P. gingivalis displays two forms of fimbriae on its surface, FimA and Mfa1, both of which are crucial for attachment to other bacteria in the oral biofilm and to the host cells. In the work presented herein we have determined the crystal structures of the shaft protein Mfa1, in both mature and precursor forms, the anchor protein Mfa2 and a truncated precursor form of the tip protein, Mfa3. The resulting mature protein thereby has an empty position in the first β-sheet that a β-strand donated from another fimbrial protein presumably fills in order to polymerize the individual proteins into a polymeric fimbria.

In order to investigate the importance of the C-terminus in terms of folding and solubility an additional construct was designed and crystallized, pMfa1Δ9, where instead the N-terminal extension was present but the final nine residues at the C-terminus were removed. pMfa1Δ9 folds into two domains, the N- and C-domain which together form an elongated structure of approximate dimensions 100 × 45 × 40 Å. The N-domain (residues 32–236) is comprised of a β-sandwich consisting of one mixed β-sheet and one anti-parallel sheet packed against each other. The C-domain (residues 237–554) also consists of two sheets, one mixed and one anti-parallel. In pMfa1Δ9 the β1-strand is anchored by the side chains of Met37, Met39, Leu41 and Met43. Further, in Mfa1 the N-terminal part of the β1-strand is shielded by a short helix that forms a lid over the sheet. In Mfa1, the β1β2 loop - where the Rgp cleavage site is located - is flexible and has not been modelled. In Mfa1, Trp554 is inserted into a hydrophobic cavity between the N- and C-terminal domains. There it forms a planar π-cation stacking interaction with Arg236 with electrostatic energy −3.68 kcal/mol, as calculated by the CaPTURE program. Arg236 is in turn firmly positioned by hydrogen bonds to Asp71 located at the end of the Nmature region. Mfa1, the shaft protein, possesses an extended C-terminus that, in the crystal structure of the mature protein, partly reaches into the void formed by the missing β1-strand. This C-terminal region, however, had to be removed in order to obtain a precursor form of Mfa1 in which the N-terminal extension is intact.

> AAKSYMSMTLSMPMGSARAGDGQDQANPDYHYVGEWAGKDKIEKVSIYMVPQGGPGLVESAEDLDFGTYYENPTIDPATHNAILKPKKGIKVNSAVGKTVKVYVVLNDIAGKAKALLANVNAADFDAKFKEIIELSTQAQALGTVADGPNPATAAGKIAKKNGTTDETIMMTCLQPSDALTIEAAVSEANAIAGIKNQAKVTVERSVARAMVSTKAQSYEIKATTQIGEIAAGSVLATITDIRWVVAQGERRQYLSKKRGTVPENTWVTPGSGFVPTSSTFHTNATEYYDYAGLWEDHNTNEAVISGTQVPTLADYQLQDVTGELANALSGKFLLPNTHKSGANAASSDYKRGNTAYVLVRAKFTPKKEAFIDRGKTYSDNTAVPEYVAGEDFFVGENGQFYVSMKSVTDPKVGGVAGMKAHKYVKGKVLYYAWLNPSTTSPDSWWNSPVVRNNIYHIHIKSIKKLGFNWNPLVPDPDPSNPENPNNPDPNPDEPGTPVPTDPENPLPDQDTFMSVEVTVLPW> AEDGPQKQQLEMPLVLDQDLTQQMRLRVESLKQRGEKKQDGEKLIRPAESVYRLDFIQQQKLQFDHW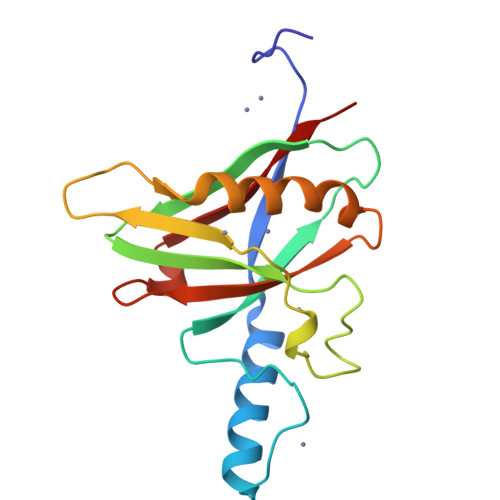NVVLDKPGKVTITGTSQNWTPDLTNLMTRQLLDPAAIFWRKEDSDAMDWNEADALEFGERLSDLAKIRKVMYFLITFGEGVEPANLKASVVFNQL> ETPPRFTRTPVDQTGVSGGVASFICQATGDPRPKIVWNKKGKKVSNQRFEVIEFDDGSGSVLRIQPLRTPRDEAIYECVASNNVGEISVSTRLTVLREDQIPRGFPTIDMGPQLKVVERTRTATMLCAASGNPDPEITWFKDFLPVDTSNNNGRIKQLRSESIGALQIEQSEESDQGKYECVATNSAGTRYSAPANLYVRVRRVPPRFSIPPTNHEIMPGGSVNITCVAVGSPMPYVKWMLGAEDLTPEDDMPIGRNVLELNDVRQSANYTCVAMSTLGVIEAIAQITVKALPKPPGTPVVTESTATSITLTWDSGNPEPVSYYIIQHKPKNSEEPYKEIDGIATTRYSVAGLSPYSDYEFRVVAVNNIGRGPASEPVLTQKHHHH;> PAPTVNTHFGKLRGARVPLPSEILGPVDQYLGVPYAAPPIGEKRFLPPEPPPSWSGIRNATHFPPVCPQNIHTAVPEVMLPVWFTANLDIVATYIQEPNEDCLYLNVYVPTEDGSGAKKQGEDLADNDGDEDEDIRDSGAKPVMVYIHGGSYMEGTGNMIDGSVLASYGNVIVITLNYRVGVLGFLSTGDQAAKGNYGLLDQIQALRWVSENIAFFGGDPRRITVFGSGIGASCVSLLTLSHHSEGLFQRAIIQSGSALSSWAVNYQPVKYTSLLADKVGCNVLDTVDMVDCLRQKSAKELVEQDIQPARYHVAFGPVIDGDVIPDDPEILMEQGEFLNYDIMLGVNQGEGLKFVEGVVDPEDGVSGTDFDYSVSNFVDNLYGYPEGKDTLRETIKFMYTDWADRDNPETRRKTLVALFTDHQWVEPSVVTADLHARYGSPTYFYAFYHHCQSLMKPAWSDAAHGDEVPYVFGVPMVGPTDLFPCNFSK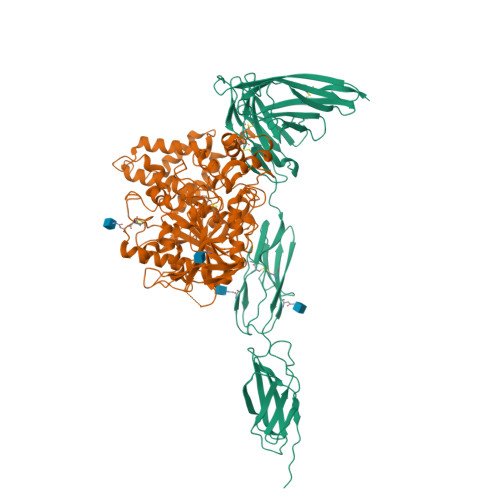NDVMLSAVVMTYWTNFAKTGDPNKPVPQDTKFIHTKANRFEEVAWSKYNPRDQLYLHIGLKPRVRDHYRATKVAFWKHLVPHLYNLHDMF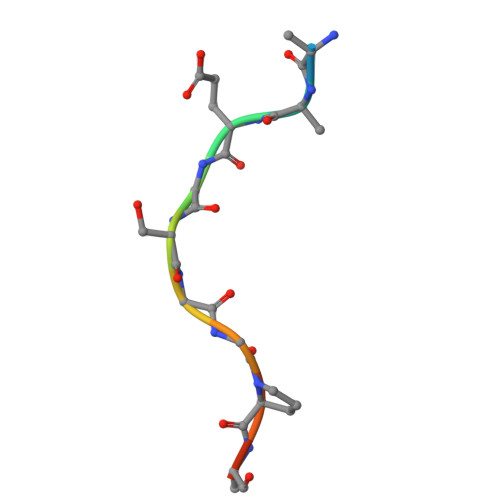> QEEEGSGGPQGG>[3x]GSHMPGPVARLAPQAVLTPPSAASLFLVLVAGDSDDDRATVCDVISGIDGPLKAVGFRELAGSLSCVVGVGAQFWDRVSASSKPAHLHPFVPLSGPVHSAPSTPGDLLFHIKAARKDLCFELGRQIVSALGSAATVVDEVHGFRYFDSRDLLGFVHGTENPTDDDAADSALIGDEDPDFRGGSYVIVQKYL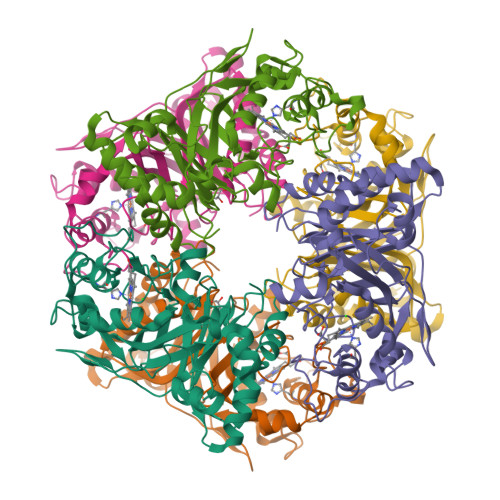HDMSAWNTLSTEEQERVIGRTKLENVELDDDAQPSNSHVTLNTIVDDDGVEHDILRDNMAFGSLGEAEYGTYFIGYAKDPAVTELMLRRMFLGEPPGNYDRVLDFSTAATGTLFFVPSRDVLESLGDEPAGAESAPEDPVEPAAAGPYDLSLKIGGLKGVSQ> MSVISIILVVLIAFLA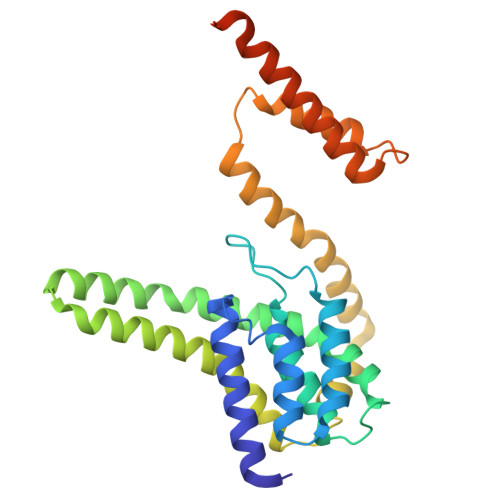GIEGILDEFQFHQPLIACTLIGLVTGNLTACIILGGTLQMIALGWANIGAAVAPDAALASVASAIILVLGGQGVAGIPSAIAIAIPLAVAGLFLTMIVRTLAVPIVHLMDRAAEKGNIRSVEWLHISAICMQGIRIAIPAAALLFIPADSVQSFLEAMPAWLTDGMAIGGGMVVAVGYALVINMMATKEVWPFFVIGFVVAAISQLTLIAIGALGVALALIYLNLSKMGGGNSNGGGGGNSRDPLGDILNDY> SNASPQPLEQIKQRESQLSGRVGMIEMDLASGRTLTAWRADERFPMMSTFKVVLCGAVLARVDAGDEQLERKIHYRQQDLVDYSPVSEKHLADGMTVGELCAAAITMSDNSAANLLLATVGGPAGLTALLRQIGDNVTRLDRWETELNEALPGDARDTTTPASMAATLRKLLTSQRLSARSQRQLLQWMVDDRVAGPLIR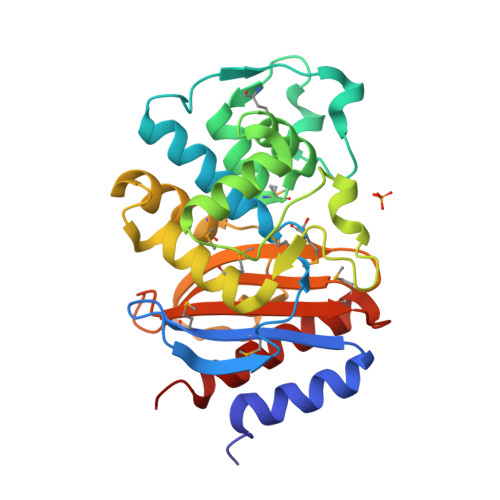SVLPAGWFIADKTGAGERGARGIVALLGPNNKAERIVVIYLRDTPASMAERNQQIAGIGAALIEHWQR(10aR)-2-(((1r,4R)-4-((2-aminoethyl)amino)cyclohexyl)methyl)-6-carboxy-4-hydroxy-4,10a-dihydro-10H-benzo[5,6][1,2]oxaborinino[2,3-b][1,4,2]oxazaborol-4-uide 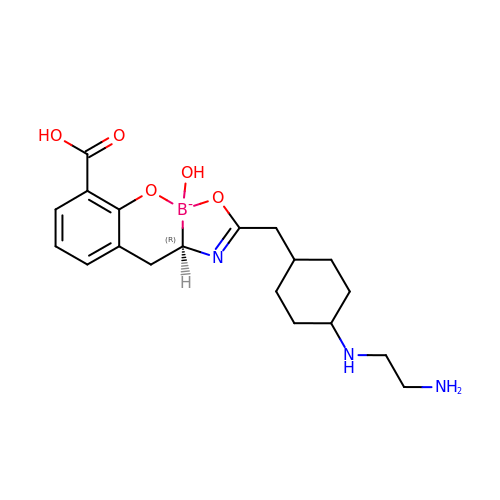| C19 H27 B N3 O5 | SXCHFKLXJGSRKQ-DXJCSPRDSA-N>[8x]MLQPPFNIKVTNITLTTAVVTWQPPILPIEGILVTFGRKNDPSDETTVDLTSSIT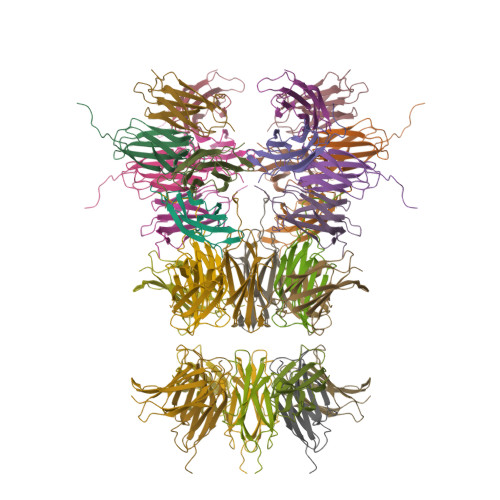SLTLTNLEPNTTYEIRIVARNGQQYSPPVSTTFTTGSLEHHHHHH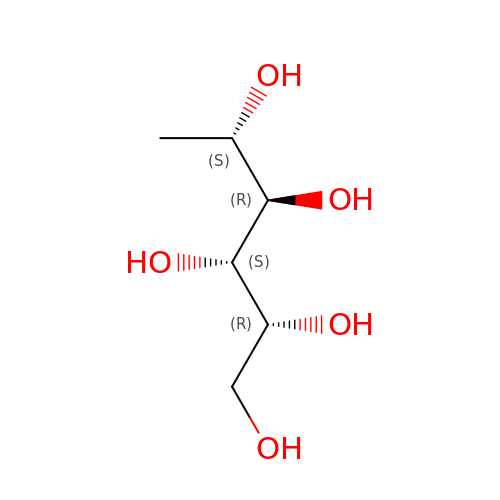FUCITOL | C6 H14 O5 | SKCKOFZKJLZSFA-KCDKBNATSA-N> MKIQKHKEIYWGELRGASISKTRKDFTYLYGSTIIFHSPDQVYFENKLIASGQTIHEWSSSWNYQGDRQVPSLPLLKRGRSYSLTRDMTSYPSESVFLKLIFF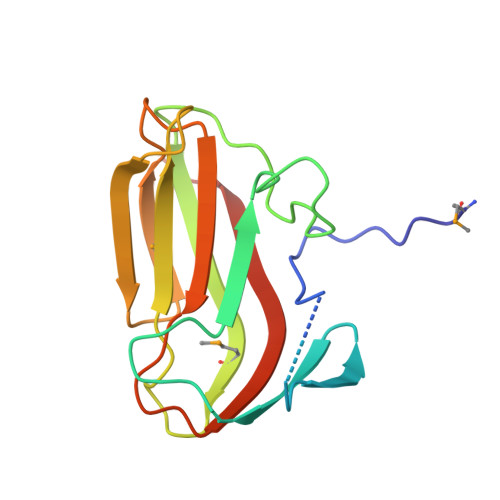DRYNREVSNHVERSDKMTFTYPEEAYSYKVQLLSAGVESFEFHCLRIEEILEESNG>GPDSMGAAAAEADRTLFVGNLETKVTEELLFELFHQAGPVIKVKIPKDKDGKPKQF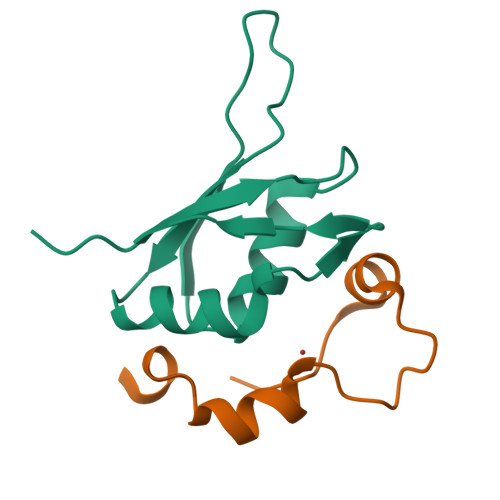AFVNFKHEVSVPYAMNLLNGIKLYGRPIKIQFRS[7x];>GPDSMRFKPGVISEELQDALGVTDKSLPPFIYRMRQLGYPPGWLK[7x]>MHHHHHHHMEQIAQQQPQTLCIKHLAKNYSKRWVVKDVSFEMQSGQIVGLLGPNGAGKTTSFYMVVGLVRMDKGEIHLDNLDLSDLAMHERARKGIGYLPQEASIFRKLTIAENIMAILETRKDLNKQQRQQRLQELLNDFKITHIKDSLGMSVSGGERRRAEIARALAADPKFMLLDEPFAGVDPISVGDIKDIIRNLKDRGIGVLITDHNVRETLAICEHAYIVSEGAVIAEGSPQDILENEQVRKVYLGDDFTV[2x];> MIIRRYLVKQVVSTSLVVIALLTLIMMGGRLIKYFGVAAQGRLDAGVLFSIIGYRMPEFLTLILPLGFFIGLMLVFGRLYVDHEMAVLNGSGISRIRLGQLLIPLALVFLVIQGILMLWMTPWGLRQFDQLSSSQAVRTGFDLVRPKEFISSGPYTIYAGDLSEDRKNLKDIFFYQRAQKEGKPDVMILAKEATRVVMENETANVVDLIQGRRYEIYPGKAKYSQAEFQRYRLRLENDKSATFETDKVEALPSSKLWNKWNDPVIASEMGWRVFGPFTIVIALMMAVALCEVSPRQGRYYRLIPAIFIFASLIVLLIAIRTRISRDELGVWAYPAALAVYGIAAALFSRKQKLAPKIKKQIKRVRA;> MLARRIVAKHVTKTTALAMLGTTIVLVILQVLFTYLGELSNLKADYSAWQAFLYVLWGAPRYLYEILPISALIGAILGLGTLASNSELIVMRSVGISLWRIVGWVIRSALVLVLLSFALSEWVVPYTNERANSVKSHQSVAALGEVRGYWSREGQRFIYVDYANSQGQLKRIQVVDFDDNYRLKSVTNAEQGQFVKDG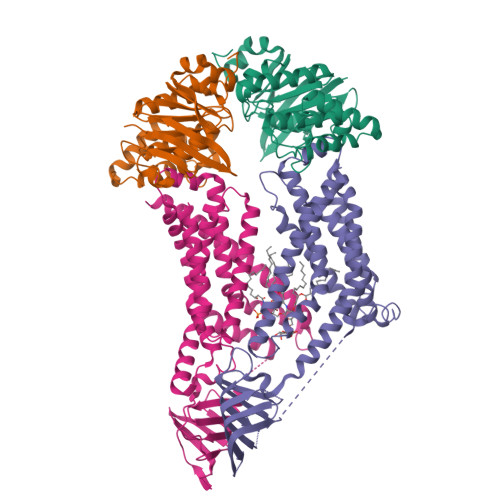QWLLNHSQQMAIQGQGDAVLANAAKQPFSLALQPKYVHMVTIDPEDLSFSQLVSFMNYMREYSQVPKTYQLAFWKKVASPFALITLVLVACSFIFGPLRQQSMGFRLVIALFIGLGFYYLQDFLGYASLVYNPSPAWFVLGPIVLMFVAGSYLLYRAR> VAFGADAAKTTQEKFDALKEAGVFSGYPGTTDAKLGQDMTRAEFAKVLVKLFGLKEIHGQYSYKDKNYDAKNWAAPFIEAVTAEGLMQAKDLTKKIFDFNGKITVEEASKTLVTALKLEPVKDAQNKATDWAKGYFEAAVNAGLFSKDANPKANATRAQLVEAAFAADEMSKGSGSHHHHHH

Prokaryotic cell envelopes often include proteinaceous surface (S-) layers composed of self-assembling subunits in porous two-dimensional crystalline lattices. S-layer anchoring is best characterized for Gram-positive bacteria, where S-layer proteins non-covalently attach to the PG layer via species- and strain-specific non-classical secondary cell wall polymers (SCWPs). SpaA possesses three consecutive SLH domains near its N-terminus, followed by a large C-terminal region presumed to harbor the self-assembling domain(s). The crystal structures and binding analyses presented here of P. alvei SpaASLH, SpaASLH/G109A, and SpaASLH/G46A/G109A with synthetic SCWP fragments provide novel insights into the functional contributions of many conserved SLH domain residues, including SLH-Trp13, SLH-Gly29, and SLH-Arg43, which precisely interlock from three different SLH domains to generate two active binding sites.

To test our hypothesis that any other amino acid would prevent the backbone flip and impede binding, a SpaASLH/G109A mutant was constructed for analyses. To confirm the structural basis for this reduced affinity, we determined the crystal structure of SpaASLH/G109A alone and in complex with 4,6-Pyr-β-d-ManNAcOMe. Unliganded SpaASLH/G109A is similar in structure to wt SpaASLH (Cα rmsd of 0.34 Å, excluding residues 44–54), and the Gly109Ala mutation is accommodated with no change in the position of Gln108 or Ala109 backbone atoms compared to Gln108 and Gly109 in the wt structure, but with a minor shift of residues 111–114. When SpaASLH/G109A crystals were soaked with 4,6-Pyr-β-d-ManNAcOMe, no electron density for ligand was observed in the resulting structures. The overall Cα rmsd between liganded and unliganded SpaASLH/G109A is 1.73 Å (1.52 Å when excluding residues 44–54), and when the SLH3 domain helices are aligned there is an 8.5 Å maximum displacement of SLH2 Cα atoms (measured for Lys91). This significant structural change explains the failure to observe ligand soaked into crystals of unliganded SpaASLH/G109A, because the structural change required for binding would not be possible in the crystal context, and also explains the initial failure to solve the complex structure by molecular replacement due to the significant difference between the search model and target structure. ITC revealed 1:1 binding to monosaccharide 4,6-Pyr-β-d-ManNAcOMe with 226 nM affinity, nearly an order of magnitude lower than the 26 nM binding observed for wt SpaASLH.> SGSPSYTENKPDKKKKYMINDAKTIQLVGPLISSPDNLGFQKRSHKARELPRFLINQEPQLEKRAFVQDPWDKANQEKMISLEESIDDLNELYETLKKMRNTERSIMEEKGLVDKADSAKDLYDAIVFQGTCLDMCPTFERSRRNVEYTVYSYEKNQPNDKKASRTKALKVFA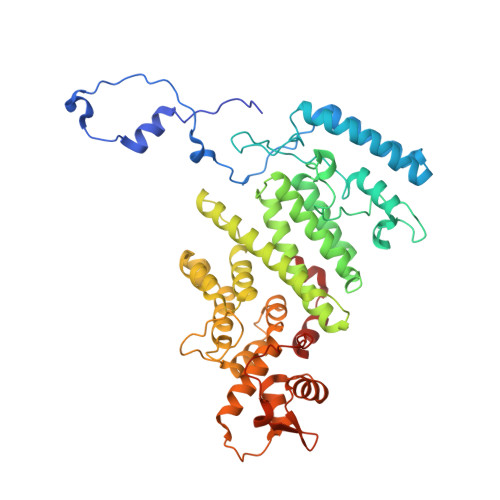RPAAAAAPPLPSDVRPPHILVKTLDYIVDNLLTTLPESEGFLWDRMRSIRQDFTYQNYSGPEAVDCNERIVRIHLLILHIMVKSNVEFSLQQELEQLHKSLITLSEIYDDVRSSGGTCPNEAEFRAYALLSKIRDPQYDENIQRLPKHIFQDKLVQMALCFRRVISNSAYTERGFVKTENCLNFYARFFQLMQSPSLPLLMGFFLQMHLTDIRFYALRALSHTLNKKHKPIPFIYLENMLLFNNRQEIIEFCNYYSIEIINGDAADLKTLQHYSHKLSETQPLKKTYLTCLERRLQKTTYKGLINGGED> TSRHKKLM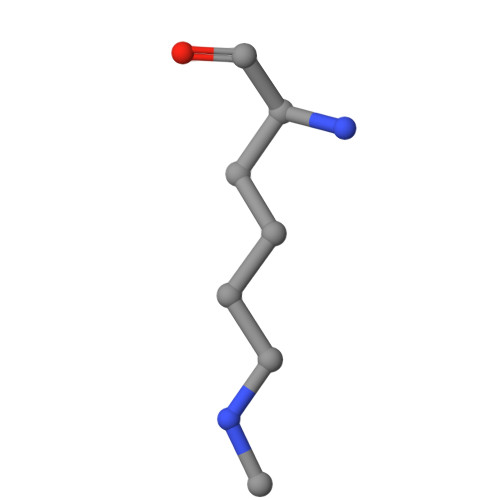FK> MAESKPTPQSTFTGPIVVDPITRIEGHLRIMVEVENGKVKDAWSSSQLFRGLEIILKGRDPRDAQHFTQRACGMCTYVHALASSRCVDDAVKVSIPANARMMRNLVMASQYLHDHLVHFYHMHALDWVDVTAALKADPNKAAKLAASIAPARPGNSAKALKAVQDKLKAFVESGQLGIFTNAYFLGGHKAYYLPPEVDLIATAHYLEALHMQVKAASAMAILGGKNPHTQFTVVGGCSNYQGLTKDPLANYLALSKEVCQFVNECYIPDLLAVAGFYKDWGGIGGTSNYLAFGEFATDDSSPEKHLATSQFPSGVITGRDLGKVDNVDLGAIYEDVKYSWYAPGGDGKHPYDGVTDPKYTKLDDKDHYSWMKAPRYKGKAMEVGPLARTFIAYAKGQPDFKKVVDMVLGKLSVPATALHSTLGRTAARGIETAI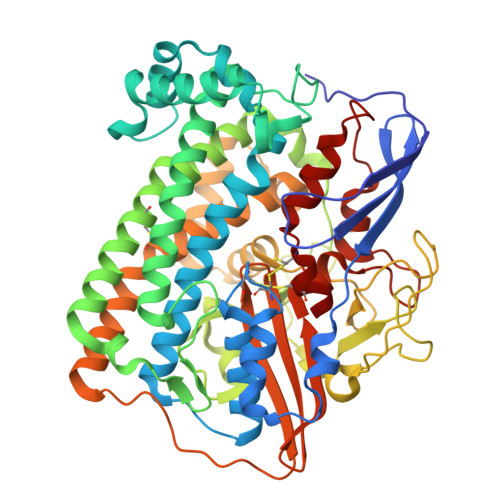VCANMEKWIKEMADSGAKDNTLCAKWEMPEESKGVGLADAPRGALSHWIRIKGKKIDNFQLVVPSTWNLGPRGAQGDKSPVEEALIGTPIADPKRPVEILRTVHAFDPCIACGVH PRPP is synthesized by PRPP synthase (PRPS), which catalyzes the transfer of diphosphate from ATP to ribose-5-phosphate (R5P), thereby generating AMP and PRPP. Class I PRPP synthase is the most widely distributed in phylogeny, including E. coli and humans. Phosphate ion (Pi) is necessary to activate class I PRPS, while ADP, an allosteric inhibitor, competes with Pi and ATP at allosteric and active sites, respectively. In both models, PRPS hexamers are stacked in rows to form filamentous polymers.

The twist and rise of type A filament are 27° (left-handed twist) and 63 Å, respectively, and the twist and rise of type B are 46° (left-handed twist) and 66 Å, respectively. Surprisingly, in type A filament, we found R5P at the active site, and the ATP binding site was occupied by ADP rather than ATP. Since we did not add ADP to the mixture for sample preparation, ADP in the model might come from the spontaneous hydrolysis of ATP or be preserved during protein purification. In type A filament, phosphate ion (Pi) binds to allosteric site 1, ADP binds to allosteric site 2 (red), and ATP binds to active site (brown). In the type A filament model, R5P and ADP at the active site are in association with two Mg2+. One Mg2+ (Mg site 1) coordinates the C1, C2, and C3 hydroxyl groups of R5P with D170 and two water molecules, and the other Mg2+ (Mg site 2) coordinates oxygens of the α- and β-phosphates of ADP (active site) with H131 and three water molecules. ADP binds allosteric site 2 in chain A through hydrogen bonding with R102 in chain B, and S149, E133 in chain A, and a π-π interaction between F147 of chain A and adenine bases, and salt bridges between R102 in chain B, R178 in chain A, and phosphates. However, in type A filaments, the RF loop is stabilized by a variety of interactions, including the salt bridge between R102 and α-phosphate of ADP at allosteric site 2, resulting in smaller B factors ranges from 29.4 to 44.5 Å2. On the other hand, the RF loop in type A filament is stabilized at a conformation and covers the ADP binding pocket at allosteric site 1.

>MPDMKLFAGNATPELAQRIANRLYTSLGDAAVGRFSDGEVSVQINENVRGGDIFIIQSTCAPTNDNLMELVVMVDALRRASAGRITAVIPYFGYARQDRRVRSARVPITAKVVADFLSSVGVDRVLTVDLHAEQIQGFFDVPVDNVFGSPILLEDMLQLNLDNPIVVSPDIGGVVRARAIAKLLNDTDMAIIDKRRPRANVSQVMHIIGDVAGRDCVLVDDMIDTGGTLCKAAEALKERGAKRVFAYATHPIFSGNAANNLRNSVIDEVVVCDTIPLSDEIKSLPNVRTLTLSGMLAEAIRRISNEESISAMFEHHHHHHH[6x]> SYS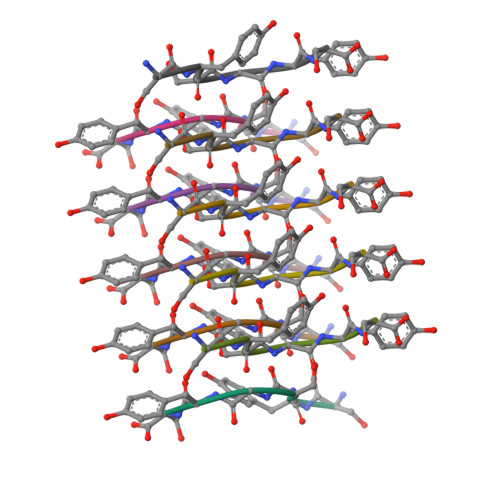GYS>MRGSHHHHHHGSMVTMEEIRRAKRAEGLATILAISTATPPNCVIQADYPDYYFGITNSEHMTELKEKFKLLCEKSMIRKRHMCLTEEILKANPNMCLYMGTSLDARQDISLVEVPKLGKEAATKAIKEWGQPKSNITHLIFCTSAGVDMPGADYQLTRLIGLNPDVKRMMIYQQGCYAGATILRLAKDLAENNKGSRVLVVCSENTIPTFRGPSYTHIDSLVGQALFADGAAALIVGADPDTSIERPLYHIVSASQTLLPDSDGAIEGHIREAGLTVHLKKDVPEFFSANIEKSLVDAFTPIGISDWNSIFWIAHPGGPAILDQVEAKLGLKKDKLRA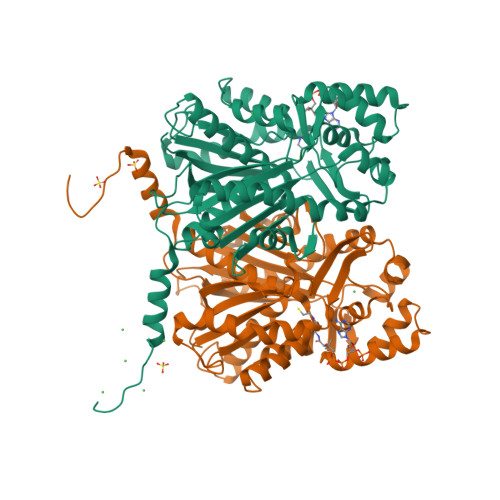SRHVMSEYGNMSSACVLFILDEMRNKCLEEGKATTGEGLDWGVLFGFGPGLTVETVVLHSLPIEA[2x]>[2x]MERAEILGVGTELLYGETLDTNTAEIARSLKPYALKVERTLRVADEVAPLAREVEEAFARARLVVLSGGLGPTPDDVTREAVALALGEPLELDEAV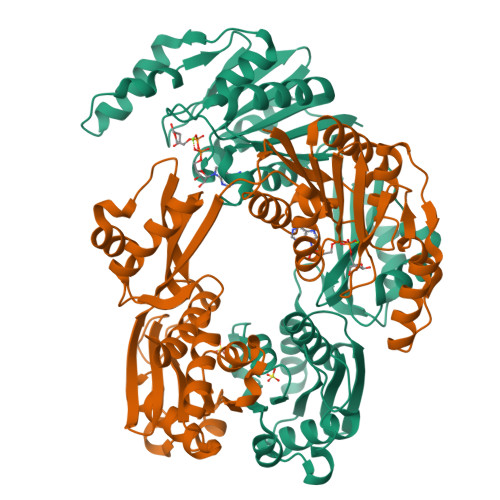LGEIEAFFRARGRAMPEANRKQAMRIPSATWLKNPRGTAPGWWVRKGGKDLVLLPGPPPEWRPMWQEVLPRLGLPRRPYAERVLKTWGIGESEIVERLGPLFVRGEEVEVGTYPKVHGVEVVVRGREDRVAELAERIKKKLLKEVWGEGEMTLAEAVKRRMEREGATLSTMESLTGGLLGAEITRVPGASRFYLGGVVSYSVGAKARFGVPQDLLSRTVSAETARAMAEAARSLFGSTYALATTGVAGPDPLEGEPPGTVYVALAGPTGAEVRRYRFPGDRETVRLRSVYAALALLVT>MTKAVHTKHAPAAIGPYSQGIIVNNMFYS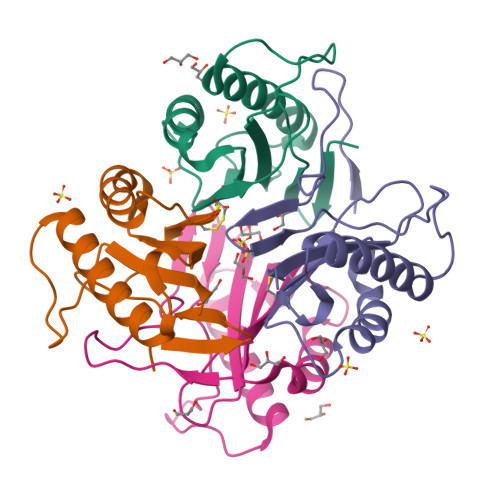SGQIPLTPSGEMVNGDIKEQTHQVFSNLKAVLEEAGASFETVVKATVFIADMEQFAEVNEVYGQYFDTHKPARFCVEVARLPKDALVEIEVIALVK[5x]>MASPIESARIGEVKRETKETNVSVKINLDGHGVSDSSTGIPFLDHMLDQLASHGLFDVHVRATGDTHIDDHHTNEDVALAIGTALLKALGERKGINRFGDFTAPLDEALIHVSLDLSGRPYLGYNLEIPTQRVGTYD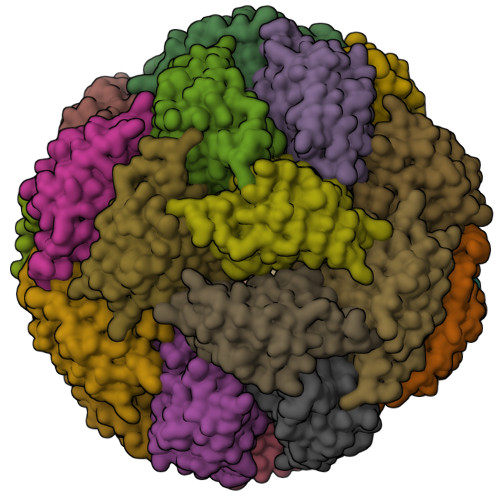TQLVEHFFQSLVNTSGMTLHIRQLAGKNSHHIIEATFKAFARALRQATESDPRRGGTIPSSKGVLSRS[24x]> GEIVSNEKSGVCINAPAKTKLQPSVFHQVFEGSKEPAVLNSKDPRLKTDFEEAIFSKYTGNKIMLMDEYMEEAVDHYVGCLEPLDISIDPIPLESAMYGMDGLEALDLTTSAGFPYLLQGKKKRDIFNRQTRDTTEMTRMLEKYGVDLPFVTFVKDELRSREKVEKGKSRLIEASSLNDSVAMRVAFGNLYATFHNNPGTATGSAVGCDPDVFWSKIPILLNGEIFAFDYTGYDASLSPVWFACLKKVL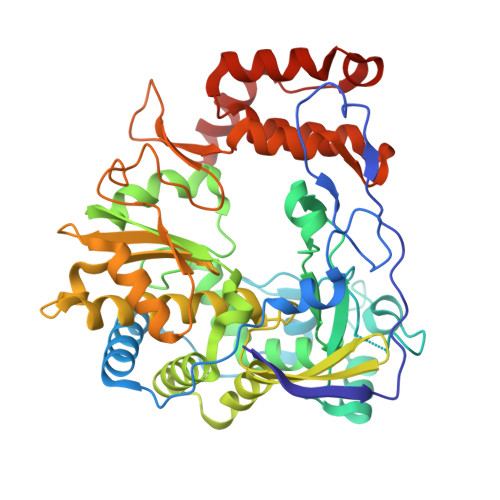IKLGYTHQTSFIDYLCHSVHLYKDRKYIVNGGMPSGSSGTSIFNTMINNIIIRTLLIRVYKGIDLDQFKMIAYGDDVIASYPHKIDPGLLAEAGKHYGLIMTPADKGTSFVDTNWENVTFLKRYFRADDQYPFLIHPVMPMKEIHESIRWTKDPRNTQDHVRSLCYLAWHNGEEAYNEFCRKIRSVPVGRALTLPAYSSLRRKWLDSF> MLNPIVRKFQYGQHTVTLETGMMARQATAAVMVSMDDTAVFVTVVGQKKAKPGQDFFPLTVNYQERTYAAGRIPGSFFRREGRPSEGETLIARLIDRPIRPLFPEGFVNEVQVIATVVSVNPQVNPDIVAMIGASAALSLSGIPFNGPIGAARVGYINDQYVLNPTQDELKESKLDLVVAGTEAAVLMVESEAELLSEDQMLGAVVFGHEQQQVVIQNINELVKEAGKPRWDWQPEPVNEALNARVAALAEARLSDAYRITDKQERYAQVDVIKSETIATLLAEDETLDENELGEILHAIEKNVVRSRVLAGEPRIDGREKDMIRGLDVRTGVLPRTHGSALFTRGETQALVTATLGTARDAQVLDELMGERTDTFLFHYNFPPYSVGETGMVGSPKRREIGHGRLAKRGVLAVMPDMDKFPYTVRVVSEITESNGSSSMASVCGASLALMDAGVPIKAAVAGIAMGLVKEGDNYVVLSDILGDEDHLGDMDFKVAGSR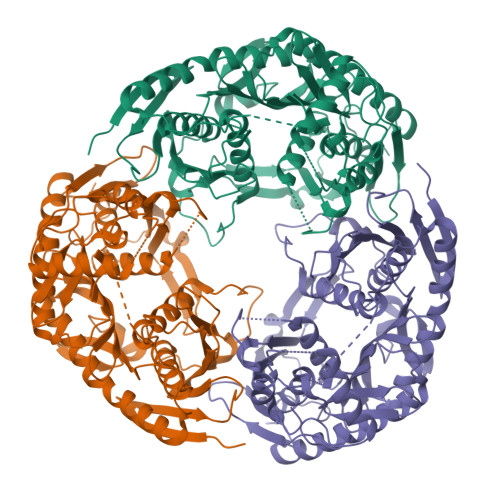DGISALQMDIKIEGITKEIMQVALNQAKGARLHILGVMEQAINAPRGDIS> VPAPGETRACGRKLISLVMAVCGDLCNPQ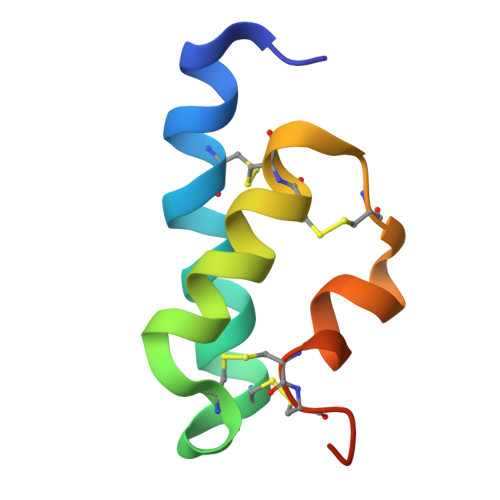EGKDIATECCGNQCSDDYIRSACCPHHHHHH(3-chloropropyl)benzene | C9 H11 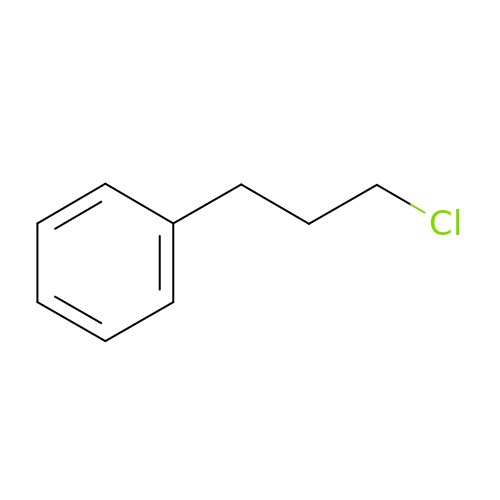Cl | XZBXAYCCBFTQHH-UHFFFAOYSA-N>GSHMDSRTVSELVTNTNTIRVAMKDAYQRDGKYPDYQAPLSLTADSIKTDSTGIAVAQLVQLGKLTPDEARNGISGDYIGIGGAITSSGSTINKGFAMELNGLSQEQCRSILGQVGDNWEYVAVGTSPSGSYDA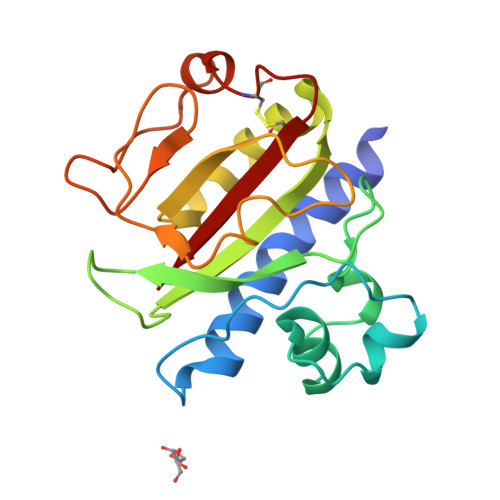LSAGAVNMLAATDNTTILRSLAANGQVSLTAEKILKTCTATVNSITLASR[2x]> NDDKLYRADSRPPDEIKQSGGLMPRGQSESFDRGTQMNINLYDHARGTQTGFVRHDDGYVSTSISLRSAHLVGQTILSGHSTYYIYVIATAPNMFNVNDVLGAYSPHPDEQEVSALGGIPYSQIYGWYRVHFGVLDEQLHRNRGYRDRYYSNLDIAPAADGYGLAGFPPEHRAWREEPWIHHAPPGCGNAPRSSMSNTCDEKTQSLGVKFLDEYQSKVKRQIFSGYQSDIDTHNRIKD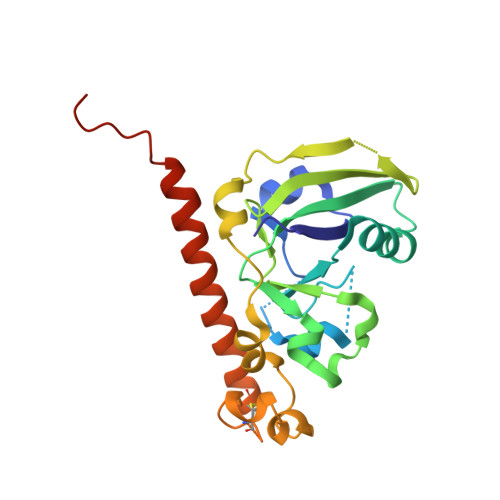EL>[10x]PGSIPLIGERFPEMEVTTDHGVIKLPDHYVSQGKWFVLFSHPADFTPVCTTEFVSFARRYEDFQRLGVDLIGLS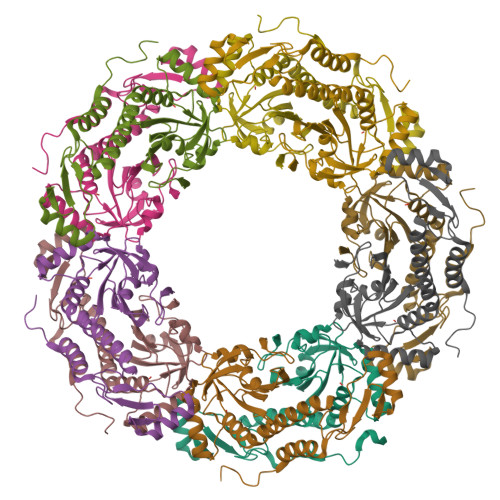VDSVFSHIKWKEWIERHIGVRIPFPIIADPQGTVARRLGLLHAESATHTVRGVFIVDARGVIRTMLYYPMELGRLVDEILRIVKALKLGDSLKRAVPADWPNNEIIGEGLIVPPPTTEDQARARMESGQYRSLDWWFCWDTPASRDDVEEARRYLRRAAEKPAKLLYEEARTHLH> SSTHPVFHMGEFSVCDSVSVWVGDKTTATDIKGKEVTVLAEVNINNSVFRQYFFETKCRASNPVESGCRGIDSKHWNSYCTTTHTFVKALTTDEKQAAW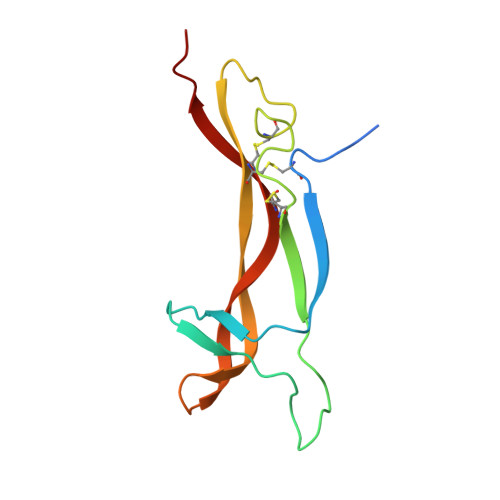RFIRIDTACVCVLSRKATR>MASMTGGQQMGRDEAGITGTWYNQLGSTFIVTAGADGALTGTYESAVGNAESRYVLTGRYDSAPATDGSGTALG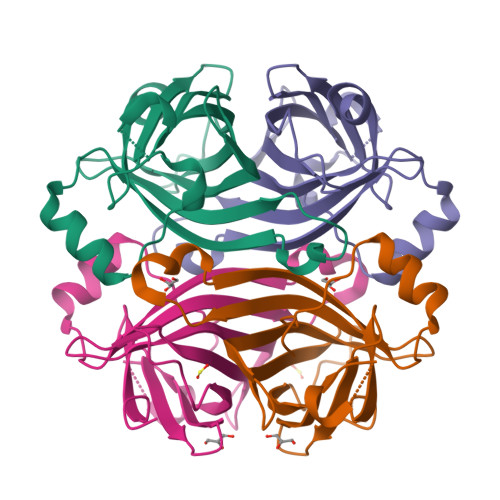WTVAWKNNYRNAHSATTWSGQYVGGAEARINTQWLLTSGTTEANAWKSTLVGHDTFTKVKPSAASIDAAKKAGVNNGNPLDAVQQ[2x]> MRTIIALETHDVRFPTSRELDGSDAMNPDPDYSAAYVVLRTDGAEDLAGYGLVFTIGRGNDVQTAAVAALAEHVVGLSVDKVIADLGAFARRLTNDSQLRWLGPEKGVMHMAIGAVINAAWDLAARAANKPLWRFIAELTPEQLVDTIDFRYLSDALTRDEALAILRDAQPQRAARTATLIEQGYPAYTTSPGWLGYSDEKLVRLAKEAV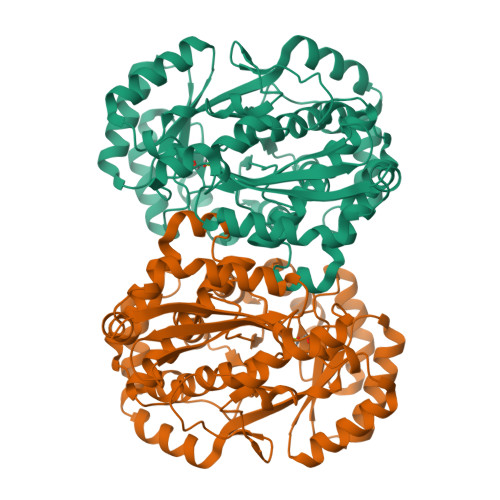ADGFRTIKLKVGANVQDDIRRCRLARAAIGPDIAMAVDANQRWDVGPAIDWMRQLAEFDIAWIEEPTSPDDVLGHAAIRQGITPVPVSTGEHTQNRVVFKQLLQAGAVDLIQIDAARVGGVNENLAILLLAAKFGVRVFPHAGGVGLCELVQHLAMADFVAITGKMEDRAIEFVDHLHQHFLDPVRIQHGRYLAPEVPGFSAEMHPASIAEFSYPDGRFWVEDLAASKAKA>[2x]SEPVTIVLSQMGWVRSAKGHDIDAPGLNYKAGDSFKAAVKGKSNQPVVFVDSTGRSYAIDPITLPSARGQGEPLTGKLTLPPGATVDHMLMESDDQKLLMASDAGYGFVCTFNDLVARNRAGKALITLPENAHVMPPVVIE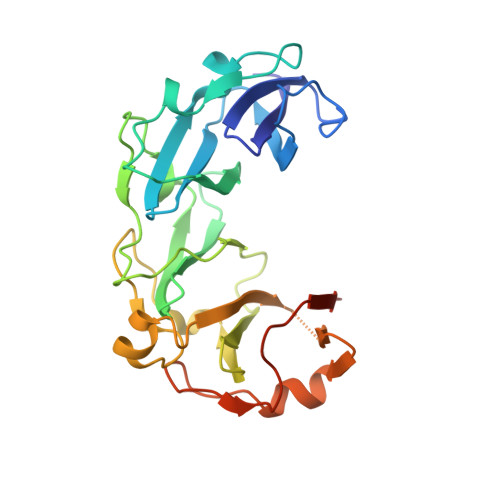DASDMLLAITQAGRMLMFPVSDLPQLSKGKGNKIINIPSAEAARGEDGLAQLYVLPPQSTLTIHVGKRKIKLRPEELQKVTGERGRRGTLMRGLQRIDRVEIDSPRRASSGDSEE>[2x]GSSKVCRGVIKLSSDCLNKMKLSDFVVLIREKYSYPQDISLLDASNQRLLFDYDFEDLNDRTLSEINLGNGSIILFSDEEGDTMIRKAIELFLDVDDELPCNTCSLPDVEVPLIKANNSPSKNEEEE;>[2x]GSMSSLCLQRLQEERKKWRKDHPFGFYAKPVKKADGSMDLQKWEAGIPGKEGTNWAGGVYPITVEYPNEYPSKPPKVKFPAGFYHPNVYPSGTICLSILNEDQDWRPAITLKQIVLGVQDLLDSPNPNSPAQEPAWRSFSRNKAEYDKKVLLQAKQYSK

The Sumo-specific E1 enzyme [the heterodimeric complex between Uba2 and Aos1 (yeast; termed Sae1-Uba2 in mammals)] initiates the process by first catalyzing adenylation of the Sumo C-terminus, which next becomes linked by a thioester bond to Uba2's catalytic cysteine. A transthiolation reaction ensues during which Sumo is transferred from Uba2 to the catalytic cysteine of the dedicated Sumo E2 conjugating enzyme, Ubc9. In addition, for both yeast and human Uba2, the ufd has been implicated in Ubc9 recruitment. Therefore, to obtain a more detailed understanding of Uba2's ufd interactions with Ubc9 and to obtain broad insights into how E1-E2 specificity is established in general, we performed structural analysis of the Uba2ufd-Ubc9 complex from S. cerevisiae.

The structure of the yeast Uba2ufd in complex with Ubc9 provides the first crystallographic insights into E1-E2 contacts in a Sumo pathway. In order to understand E1-E2 interactions in a Sumo pathway, we determined the crystal structure of a Uba2ufd-Ubc9 complex from yeast. There are two molecules per asymmetric unit, which superimpose with 0.3 Å root mean square deviation (rmsd) over all alpha carbons, so only one version of the complex is discussed here. The structure of Ubc9 superimposes well with the prior structure of free Ubc9 (0.55 Å rmsd), with the most notable difference being slight variation in the position of the β1β2-loop. The Uba2ufd-Ubc9 interface is interdigitated, with the two V-shaped grooves from Uba2 binding alternating regions of Ubc9, as in a layered sandwich. Ubc9's Lys30 from one face of the β1β2-loop forms a salt-bridge with Uba2's Asp493. On the other side, Ubc9's Asp33 interacts with Uba2's Arg484. Ubc9's Met36 and Leu38, at the C-terminus of the β1β2-loop, pack against a hydrophobic ridge comprising Uba2's Leu478, Leu485, and Phe491 in the first “V”. The complex structure also provides only the second detailed view of E1ufd-E2 interactions for any UBL, and demonstrates a common overall mode of E2 recruitment by E1 ufds: a ufd's “W” (i.e., double-“V”) -shaped surface engages an E2's N-terminal helix and β1β2-loop. Finally, docking the Uba2ufd-Ubc9 structure on prior structures of full-length Uba2 indicate that the Uba2 ufd would need to undergo significant rotation so that the Uba2 and Ubc9 cysteines could face each other.>GHMSLGSQKERLLDELTLEGVARYMQSERCRRVICLVGAGISTSAGIPDFRSPSTGLYDNLEKYHLPYPEAIFEISYFKKHPEPFFALAKELYPGQFKPTICHYFMRLLKDKGLLLRCYTQNIDTLERIAGLEQEDLVEAHGTFYTSHCVSASCRHEYPLSWMKEKIFSEVTPKCEDCQSLVKPDIVFFGESLPARFFSCMQSDFLKVDLLLVMGTSLQVQPFASLISKAPLSTPRLLINKEKAGQSDPFLGMIMGLGGGMDFDSKKAYRDVAWLGECDQ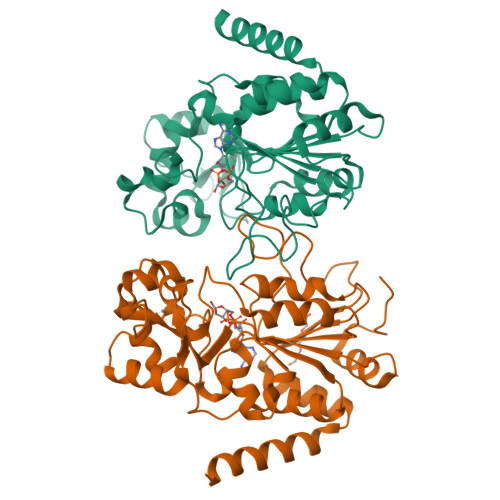GCLALAELLGWKKELEDLVRREHASIDAQS[2x]(3R)-N-benzylpyrrolidin-3-amine | C11 H16 N2 | 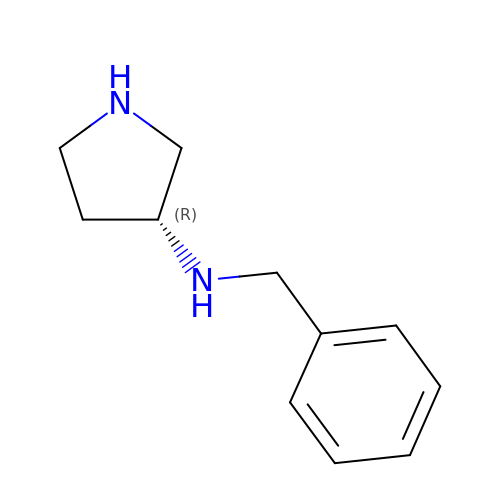NFLXIAUKMQBTMN-LLVKDONJSA-N> MILDTDYITEDGKPVIRIFKKENGEFKIDYDRNFEPYIYALLKDDSAIEDVKKITAERHGTTVRVVRAEKVKKKFLGRPIEVWKLYFTHPQDQPAIRDKIKEHPAVVDIYEYDIPFAKRYLIDKGLIPMEGDEELKMLAFAIATLYHEGEEFAEGPILMISYADEEGARVITWKNIDLPYVDVVSTEKEMIKRFLKVVKEKDPDVLITYNGDNFDFAYLKKRSEKLGVKFILGREGSEPKIQRMGDRFAVEVKGRIHFDLYPVIRRTIWLPTYTLEAVYEAIFGQPKEKVYAEEIAQAWETGEGLERVARYSMEDAKVTYELGKEFFPMEAQLSRLVGQSLWDVSRSSTGNLVEWFLLRKAYERNELAPNKPDERELARRRESYAGGYVKEPERGLWENIVYLDFRSLYPSIIITHNVSPDTLNREGCGEYDVAPQVGHKFCKDFPGFIPSLLGPLLEERQKVKKKMKATIDPIEKKLLDYRQRLIGILANSFYGYYGYAKARWYCKECAESVTAWGRQYLETTIREIEEKFGFKVLYADTDGFFATIPGADAETVKKKAKEFLDYINAKLPGLLELEYEGFYKRGFFATK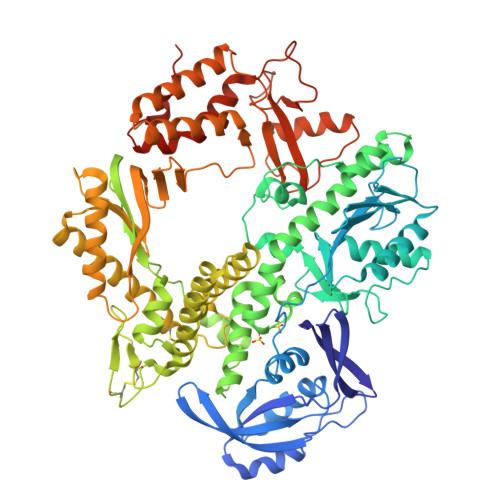KKYAVIDEEDKITTVGLEIVRVDWSEIAKETQARVLEAILKHGDVEEAVRIVKEVTEKLSKYEVPPEKLVIYEQITRDLKDYKATGPHVAVAERLAARGIKIRPGTVISYIVLKGSGRIGDRAIPFDEFDPAKHRYDAEYYIENQVLPAVERILRAFGYRKEDLRYQKTRQVGLGAWLKPKT>[4x]SGSPEFNMAAKLEVREAMLTEKRVCRF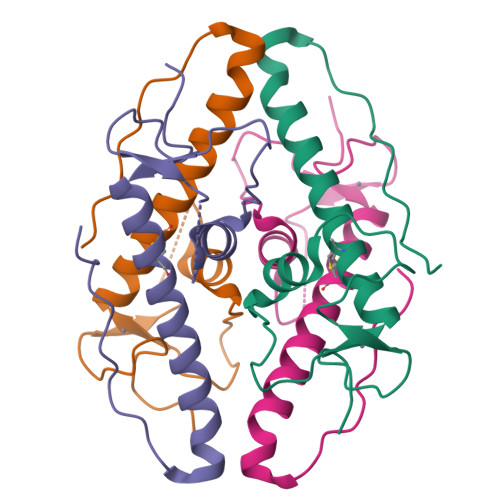CLTEQKLASIFEENPRVKTTANLPLQIMAITAIEVYAGDGMPGHICLECRLLFEHCYRFKQMCKRAETLLRQYPLTGNWPSPLEKPRAPISS> MSVSVVVPSAKATGAGGKKAKTFKVIKVSTPKVNNVHVPK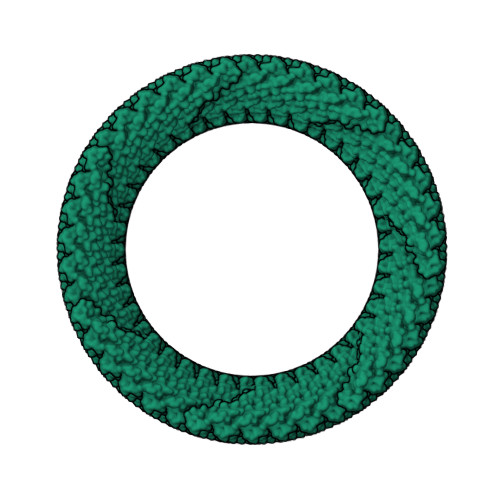IKKATRIHDPGAISGSLAKVTFGTNGFDIPTIAIALLIVGVIIGLSGLILSIFATATASAISNPSPGTLAYNLTHPLINGMVSFFSFFPTLYVLLGVTGIVLIAAGIISIIMEKFKT> KHPTPMLDELEKGPWPSFVSDIKQECDNRAKNPKGLDYQIPAECPDDLLGILELSFHEGETHWKHGGIVGVFGYGGGVIGRYCDQPEM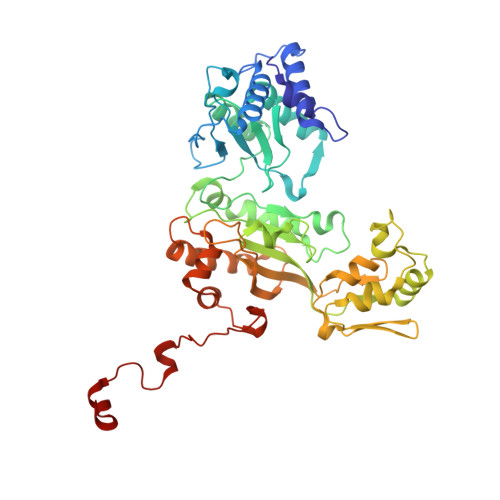FPGVAHFHTVRLAQPAAKYYTAEYLEAICDVWDLRGSGLTNMHGSTGDIVLLGTQTPQLEEIFFEMTHNLNTDLGGSGSNLRTPESCLGISRCEFACYDTQLMCYQLTQDYQDELHRPAFPYKFKFKFDGCPNGCVASMARSDFAVIGTWKDDIKIDQEAVKAYVGGEFKPNAGAHAGRDWGKFDIEAEVVGLCPTGCMTYESGTLSIDNKNCTRCMHCINTMPRALKIGDERGASILVGAKAPVLDGAQMGSLLIPFIAAEEPFDEVKEVIENIWEWWMEEGKNRERLGETMKRVGFQKLLEVTGTKAVPQHVSEPRHNPYIFFKEEEVPGGWSRDISDYRKRHMR> MRAEGLGGLERFCSPGKGRGLRALQPFQVGDLLFSCPAYAYVLTVNERGNHCEYCFTRKEGLSKCGRCKQAFYCNVECQKEDWPMHKLECSPMVVFGENWNPSETVRLTARILAKQKIHPERTPSEKLLAVKEFESHLDKLDNEKKDLIQSDIAALHHFYSKHLGFPDNDSLVVLFAQVNCNGFTIEDEELSHLGSAIFPDVALMNHSCCPNVIVTYKGTLAEVRAVQEIKPGEEVFTSYIDLLYPTEDRNDRLRDSYFFTCECQECTTKDKDKAKVEIRKLSDPPKAEAIRDMVRYA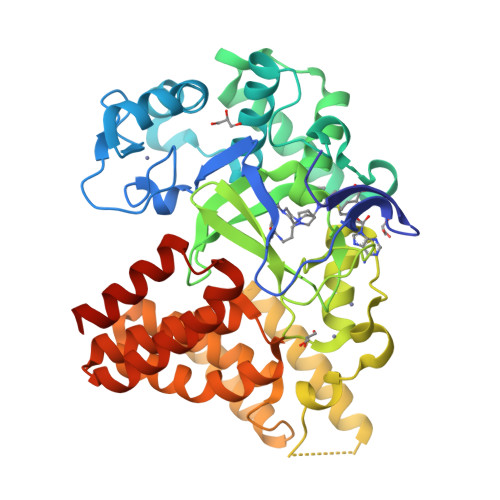RNVIEEFRRAKHYKSPSELLEICELSQEKMSSVFEDSNVYMLHMMYQAMGVCLYMQDWEGALQYGQKIIKPYSKHYPLYSLNVASMWLKLGRLYMGLEHKAAGEKALKKAIAIMEVAHGKDHPYISEIKQEIESHEGHHHHHH The Mononegavirales order groups five families of monopartite, negative-strand RNA viruses many of which are highly pathogenic and/or contagious; the Filoviridae (of which Ebola virus is a representative), the Bornaviridae (Borna disease virus), the Nyamiviridae (midway virus), the Rhabdoviridae (rabies, vesicular stomatitis virus (VSV)) and the Paramyxoviridae (measles virus, human metapneumovirus (hMPV)). These viruses encode a large RNA polymerase (L) (usually >2,000 amino acids) that is crucial to viral replication. As a part of this study, we expressed CR-VI+, a 406-residue fragment comprising CR-VI and the adjoining ‘+ domain’, the variable region carrying the K-K-G-motif, investigated its MTase activity and solved its crystal structure. Besides sequentially methylating the 2′O and N7 atoms of small capped RNAs, CR-VI+ also 2′O methylates uncapped substrates and displays nucleotide triphosphatase (NTPase) activity. Both the CR-VI domain, which assumes a fairly standard MTase fold, and the K-K-G motif of the (mainly helical) +domain are required for the MTase reactions.

In crystals of the monomeric C1877A mutant (space group P3121), this disordered, unstable region is further enlarged, as helix α+2 completely unfolds and α+3 unwinds to 3½ turns.

> MALLTPIPSPMVNLTQVIDPTEQLAYFPKITFERLKNYDTSSNYAKGKLTRNYMILLPWQHVNRYNFVFSSTGCKVSLKTCIGKLMKDLNPKVLYFIGEGAGNWMARTACEYPDIKFVYRSLKDDLDHHYPLEYQRVIGELSRIIDSGEGLSMETTDATQKTHWDLIHRVSKDALLITLCDAEFKDRDDFFKMVILWRKHVLSCRICTTYGTDLYLFAKYHAKDCNVKLPFFVRSVATFIMQGSKLSGSECYILLTLGHHNNLPCHGEIQNSKMKIAVANDFYAAKKLDNKSIEANCKSLLSGLRIPINKKELNRQRRLLTLQSNHSSVATVGGSKVIESKWLTNKANTIIDWLEHILNSPKGELNYDFFEALENTYPNMIKLIDNLGNAEIKKLIKVTGYMLVSKKSGHHHHHH>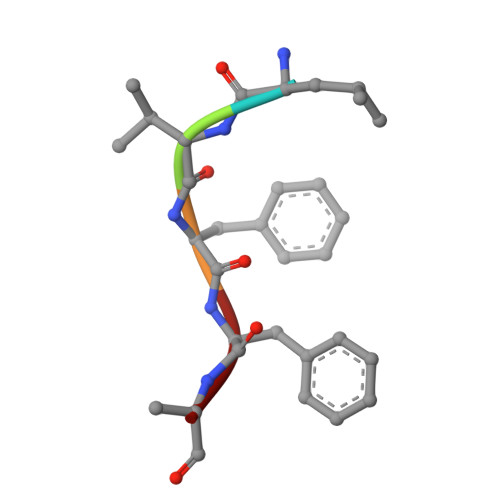 LVFFA> GAHMGNWATHVYVPYEAKEE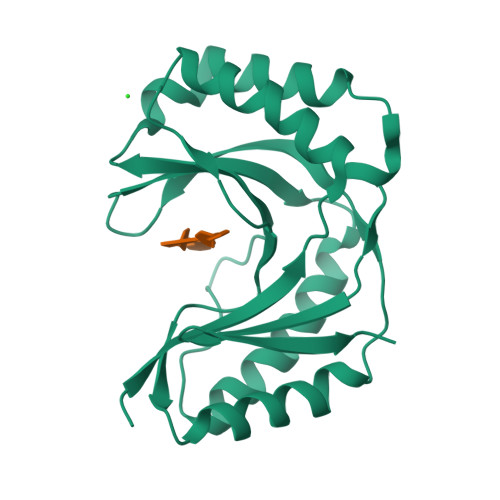FLDLLDVLLPHAQTYVPRLVRMKVFHLSLSQSVVLRHHWILPFVQALKARMTSFHRFFFTANQVKIYTNQEKTRTFIGLEVTSGHAQFLDLVSEVDRVMEEFNLTTFYQDPSFQLSLAWCVGDARLQLEGQCLQELQAIVDGFEDAEVLLRVHTEQVRCKSGNKFFSMPLK> MQRTLRSAARRKWGQKTWSPTATNGGAAPANGVSAQEALQIAYRPMPPSQTVEYEEDFGH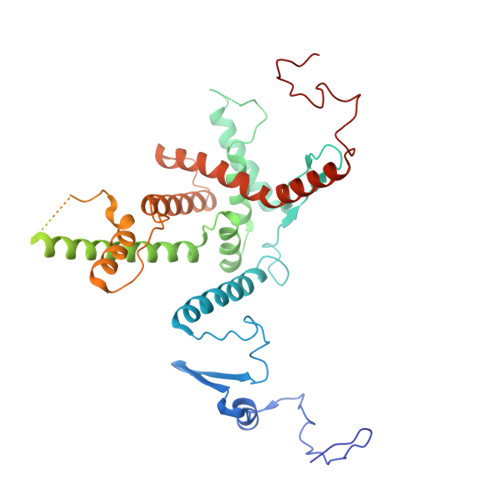NLMIHREYISKRCRDRVSFELSALSYSNLELRRGQEHLAGIMNRERRGVSVGASGAPDDQVQMQTDVDANSREVLSARYLFNERRLQFCDRFQNFFQSKLENSAASDSNGHEKQHLFSLMEACAVIFGCETEAARETYYRMFLGLDSETLLEEDEALRNRIADAKLVQRVLENNKGRQEVTQSPKLQQQQDQGKPLHAVSSGTSLLNDCEEERFISSIPELSLFEDETEARANGFVEGEDDVKANNGDLTAGSFSSPASSVNLPEEFEEYAPLYKAYITHAVGKGPVASYDISTLGSTGLTAERRRWRTLMEKIVREDYHTMTEVEQMDAIVLNEQLHTVKFFDLKIGDAIRDILQLLQRETGVGSSVNRDTPVGISPNNPERRV MICALs are a phylogenetically conserved family of actin regulatory enzymes that bind and disassemble actin filaments (F-actin). In particular, MICALs bind directly to F-actin and stereospecifically oxidize two conserved methionine residues (Met44 and Met47) into methionine sulfoxides. MICALs are large, multidomain intracellular proteins. The MO non-covalently binds the FAD cofactor and uses NADPH and oxygen to drive its oxidative mechanisms.

We determined the structure of the human MICAL1 using single-particle cryo-EM to a nominal resolution of 3.1 Å. The cryo-EM density map was clearly defined for all four domains but less visible for the linker regions, which were not built into the model. Analogous to its murine counterpart, the human MO domain comprises two subdomains of distinct sizes interconnected by two beta-strands (MOβ9 and MOβ15). A deep cavity located between these subdomains is partially occupied by the FAD cofactor, which, in the cryo-EM structure, is observed in its oxidized state with the isoalloxazine ring in a planar conformation. The interaction between the MO and CC domains is primarily mediated by the CCα1 helix, wedged within a shallow cavity between the large and small subdomains of the MO. The interface between the MO and CC domains is extensive, burying a total solvent-accessible area of 2554 Å2. A key feature of the MO-CC interaction involves a region between MOβ17 and MOα15, potentially acting as a molecular switch. This region includes Trp400, which stabilizes the FAD’s isoalloxazine ring through coaxial stacking, and adjacent Phe399, stabilizing the MO-CC interaction via a cation-π interaction with Arg933 from the CCα1 helix. In the cryo-EM structure, the CH domain binds to the CC domain. The LIM domain engages the central part of the CCα1 and CCα2 mainly through hydrophobic contacts. Given the high quality of the cryo-EM density in this region, we confidently modeled this helix within the L2 linker (residues 630–647), which we have labeled L2α1. This helix is wedged between the CC, CH, and LIM domains and plays a crucial role in the stability of the CH-LIM-CC assembly. Interestingly, the opposite face of the MO domain, which contains the deep cavity housing the FAD cofactor, exhibited minimal changes in deuteration, except for a minor helical region spanning residues 201-206. These observations suggest that the binding site for the CCα1inh helix on the MO domain partially or fully overlaps with the F-actin binding site.

> MASPTSTNPAHAHFESFLQAQLCQDVLSSFQELCGALGLEPGGGLPQYHKIKDQLNYWSAKSLWTKLDKRAGQPVYQQGRACTSTKCLVVGAGPCGLRVAVELALLGARVVLVEKRTKFSRHNVLHLWPFTIHDLRALGAKKFYGRFCTGTLDHISIRQLQLLLLKVALLLGVEIHWGVTFTGLQPPPRKGSGWRAQLQPNPPAQLANYEFDVLISAAGGKFVPEGFKVREMRGKLAIGITANFVNGRTVEETQVPEISGVARIYNQSFFQSLLKATGIDLENIVYYKDDTHYFVMTAKKQCLLRLGVLRQDWPDTNRLLGSANVVPEALQRFTRAAADFATHGKLGKLEFAQDAHGQPDVSAFDFTSMMRAESSARVQEKHGARLLLGLVGDCLVEPFWPLGTGVARGFLAAFDAAWMVKRWAEGAESLEVLAERESLYQLLSQTSPENMHRNVAQYGLDPATRYPNLNLRAVTPNQVRDLYDVLAKEPVQRNNDKTDTGMPATGSAGTQEELLRWCQEQTAGYPGVHVSDLSSSWADGLALCALVYRLQPGLLEPSELQGLGALEATAWALKVAENELGITPVVSAQAVVAGSDPLGLIAYLSHFHSAFKSMAHSPGPVSQASPGTSSAVLFLSKLQRTLQRSRAKENAEDAGGKKLRLEMEAETPSTEVPPDPEPGVPLTPPSQHQEAGAGDLCALCGEHLYVLERLCVNGHFFHRSCFRCHTCEATLWPGGYEQHPGDGHFYCLQHLPQTDHKAEGSDRGPESPELPTPSENSMPPGLSTPTASQEGAGPVPDPSQPTRRQIRLSSPERQRLSSLNLTPDPEMEPPPKPPRSCSALARHALESSFVGWGLPVQSPQALVAMEKEEKESPFSSEEEEEDVPLDSDVEQALQTFAKTSGTMNNYPTWRRTLLRRAKEEEMKRFCKAQTIQRRLNEIEAALRELEAEGVKLELALRRQSSSPEQQKKLWVGQLLQLVDKKNSLVAEEAELMITVQELNLEEKQWQLDQELRGYMNREENLKTAADRQAEDQVLRKLVDLVNQRDALIRFQEERRLSELALGTGAQG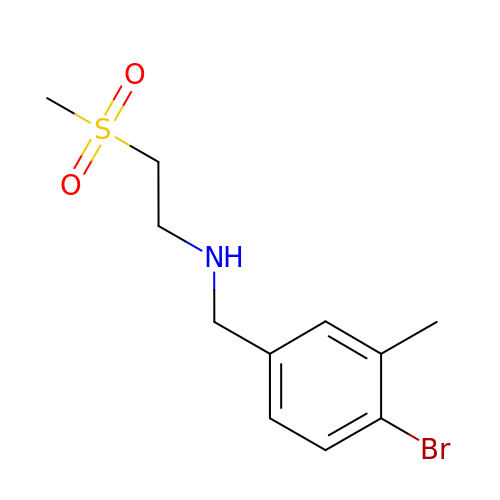N-[(4-bromo-3-methylphenyl)methyl]-2-(methylsulfonyl)ethan-1-amine | C11 H16 Br N O2 S | ODRAFWBQWMPBEH-UHFFFAOYSA-N The otopetrin (OTOP) proteins were recently characterized as extracellular proton-activated proton channels. Several recent OTOP channel structures demonstrated that the channels form a dimer with each subunit adopting a double-barrel architecture. In this study, we performed structural and functional characterization of the Caenorhabditis elegans OTOP8 (CeOTOP8) and mouse OTOP2 (mOTOP2) and illuminated a set of conformational changes related to the proton-conducting process in OTOP. Combining the structural information from both channels, we propose a working model describing the multi-step conformational changes during the proton conducting process.

Mouse OTOP2 was expressed in HEK293F cells and purified in glyco-diosgenin (GDN) detergent. Its single-particle cryo-EM structures were determined using protein samples prepared at various pH conditions (5.0, 7.0, 8.0, and 9.0). The structure from the major group of particles (3.22 Å) is similar to that determined at pH 5.0 (3.06 Å). Among all, the mOTOP2 structures determined at pH 5.0 and 8.0 are better resolved and will be used to represent the low and high pH structures, respectively, in the following discussion. The structure difference in mOTOP2 between low and high pH conditions is quite subtle and mainly occurs at the N-terminal half of TM6 preceding the highly conserved glutamate (Glu250 in mOTOP2) important for proton transfer. At low pH, TM6 of mOTOP2 forms a bent helix with a kink at Pro246 just one helical turn above Glu250 whose side chain, likely in a protonated state, is pinned to the center of the hydrophobic interface between the N- and C-barrels (left insets). In mOTOP2, however, the two equivalent residues (Glu250 and His551) are too far apart (with Cβ-to-Cβ distances of about 14.8 Å at high pH and 12.8 Å at low pH) to form a similar proton-transferring bridge by a simple side-chain movement, suggesting that conformational change is required to move them closer before they can engage in proton transfer. Firstly, the helix-to-loop transition at the N-terminal part of TM6 observed in mOTOP2 determines whether the glutamate is exposed to the extracellular solution for protonation or buried in the inter-barrel interface in a protonated state ready to contribute its proton to an acceptor. Once protonated, the loop-to-helix transition at the N-terminus of TM6 drives the proton-carrying glutamate side chain to the middle of the inter-barrel interface as depicted in state 2. The two conformations observed in mOTOP2 structures represent these first two states of the proton-conducting process, whereas the CeOTOP8 structures likely capture the next two states (states 3 and 4).

>MSEELVPHPNESLPGPRASPREVWKKGGRLLSVLLAVNVLLLACTLISGGAFNKVAVYDTDVFALLTTMMLLAALWIVFYLLRTARCPDAVPYRDAHAGPIWLRGGLVLFGICTLVMDVFKTGYYSSFFECQSAIKILHPIIQAVFVIVQTYFLWISAKDCIHTHLDLTRCGLMFTLATNLAIWMAAVVDESVHQAHSYSGSHGNTSHTRLNPDSKRAGGAAEEDPCLCSTAICQIFQQGYFYLYPFNIEYSLFASTMLYVMWKNVGRLLASTHGHGHTPSRVSLFRETFFAGPVLGLLLFVVGLAVFILYEVQVSGERGHTRQALVIYYSFNIVCLGLMTLVSLSGSVIYRFDRRAMDHHKNPTRTLDVALLMGAALGQYAISYYSIVAVVVGSPRDLQGALNLSHALLMIAQHTFQNVFIIESLHRGPPGAEPREMPPKEPCQGITFANLDAIRTLPSCPPTPRLVIPNLESPQEAVAIISAPRCHWRRRCLKDISLFLLLCNVILWIMPAFGARPHFSNTVEVDFYGYSLWAAIVNICLPFGIFYRMHAVSSLLEVYVLS[2x]>[2x]MEAFEISDFKEHAKKKSMWAGALNKVTISGLMGVFTEDEDLMALPIHRDHCPALLKIFDEIIVNATDHERACHNKTKKVTYIKISFDKGVFSCENDGPGIPIAKHEQASLIAKRDVYVPEVASCHFLAGTNINKAKDCIKGGTNGVGLKLAMVHSQWAILTTADGAQKYVQHINQRLDIIEPPTITPSREMFTRIELMPVYQELGYAEPLSETEQADLSAWIYLRACQCAAYVGKGTTIYYNDKPCRTGSVMALAKMYTLLSAPNSTIHTATIKADAKPYSLHPLQVAAVVSPKFKKFEHVSVINGVNCVKGEHVTFLKKTINEMVVKKFQQTIKDKNRKTTLRDSCSNIFIVIVGSIPGIEWTGQRKDELSIAENVFKTHYSIPSSFLTSMTKSIVDILLQSISKKDNHKQVDVDKYTRARNAGGKRAQDCMLLAAEGDSALSLLRTGLTLGKSNPSGPSFDFCGMISLGGVIMNACKKVTNITTDSGETIMVRNEQLTNNKVLQGIVQVLGLDFNCHYKTQEERAKLRYGCIVACVDQDLDGCGKILGLLLAYFHLFWPQLIIHGFVKRLLTPLIRVYEKGKTMPVEFYYEQEFDAWAKKQTSLANHTVKYYKGLAAHDTHEVKSMFKHFDNMVYTFTLDDSAKELFHIYFGGESELRKRELCTGVVPLTETQTQSIHSVRRIPCSLHLQVDTKAYKLDAIERQIPNFLDGMTRARRKILAGGVKCFASNNRERKVFQFGGYVADHMFYHHGDMSLNTSIIKAAQYYPGSSHLYPVFIGIGSFGSRHLGGKDAGSPRYISVQLASEFIKTMFPAEDSWLLPYVFEDGQRAEPEYYVPVLPLAIMEYGANPSEGWKYTTWARQLEDILALVRAYVDKDNPKHELLHYAIKHKITILPLRPSNYNFKGHLKRFGQYYYSYGTYVISEQRNIITITELPLRVPTVAYIESIKKSSNRMTFIEEIIDYSSSETIEILVKLKPNSLNRIVEEFKETEEQDSIENFLRLRNCLHSHLNFVKPKGGIIEFNTYYEILYAWLPYRRELYQKRLMREHAVLKLRIIMETAIVRYINESAELNLSHYEDEKEASRILSEHGFPPLNHTLIISPEFASIEELNQKALQGCYTYILSLQARELLIAAKTRRVEKIKKMQARLDKVEQLLQESPFPGASVWLEEIDAVEKAIIKGRNTQWKFH

The viral type II topoisomerase encoded by the African swine fever virus (ASFV) is critical for viral replication and infection, thus representing an attractive target for antiviral drug development. Type II topoisomerases can relax supercoiled DNA by a concerted strand-passage mechanism in which the enzyme first cleaves one DNA duplex (G-segment) and then guides the second DNA duplex (T-segment) to pass through the transient breaks. ASFV P1192R contains two conserved domains, namely, an N-terminal ATPase domain and a central DNA cleavage core followed by a coiled-coil arm, but lacks the nonconserved C-terminal domain (CTD) with modulating activities reported in human topo II. Similar to previously reported topo II structures of yeast and human, P1192R assembles into a large homodimer mediated by two interfaces.

Interestingly, 3D classification revealed two distinct classes with almost even particle populations, generating high-resolution reconstructions with C2 symmetry imposed at an overall resolution of 3.16 Å and 3.13 Å, respectively. One state has a closed conformation in the C-terminal dimer interface, and the other one appears open. In our study, two distinct P1192R dimeric states were observed simultaneously in the cryo-EM samples, with their DNA-gate closed, whereas their C-gate is closed and open, respectively. It shows that the conformations of the DNA cleave core for the two P1192R dimers are nearly identical, with a root-mean-square deviation (RMSD) value of 1.25 Å for all Cα. However, the coiled-coil arm of the closed state rotates inward by ~15° relative to that of the open state, thus leading to an enclosed C-gate interface stabilized via extensive intermolecular hydrogen bond and ionic interactions. Compared with the yeast topo II, P1192R contains an additional pair of E817-R1046 salt bridge, which is retained in the closed state while disrupted in the open state. Since no DNA substrates are present in the cryo-EM samples, we consider that the C-gate could adopt both closed and open conformations prior to reaction, and its status might be self-regulated through inter-domain interactions. In our study, we observed that the P1192R simultaneously exists in two states in solution, with its C-gate closed or open, providing the first experimental evidence to support the previously proposed model. The N-terminal ATPase domain comprising amino acids 1–414 was invisible in both states, probably owing to its flexible connection with the other part of P1192R. Besides the ATPase domain, the cryo-EM densities corresponding to the region covering residues 471–501 also could not be traced in these two states.>[8x]MGSSHHHHHHSSGRENLYFQGMELLKHLSQRQYIDGEWVESANKNTRDIINPYNQEVIFTVSEGTKEDAERAILAARRAFESGEWSQETAETRGKKVRAIADKIKEHREALARLETLDTGKTLEESYADMDDIHNVFMYFAGLADKDGGEMIDSPIPDTESKIVKEPVGVVTQITPWNYPLLQASWKIAPALATGCSLVMKPSEITPLTTIRVFELMEEVGFPKGTINLILGAGSEVGDVMSGHKEVDLVSFTGGIETGKHIMKNAANNVTNIALELGGKNPNIIFDDADFELAVDQALNGGYFHAGQVCSAGSRILVQNSIKDKFEQALIDRVKKIKLGNGFDADTEMGPVISTEHRNKIESYMDVAKAEGATIAVGGKRPDRDDLKDGLFFEPTVITNCDTSMRIVQEEVFGPVVTVEGFETEQEAIQLANDSIYGLAGAVFSKDIGKAQRVANKLKLGTVWINDFFM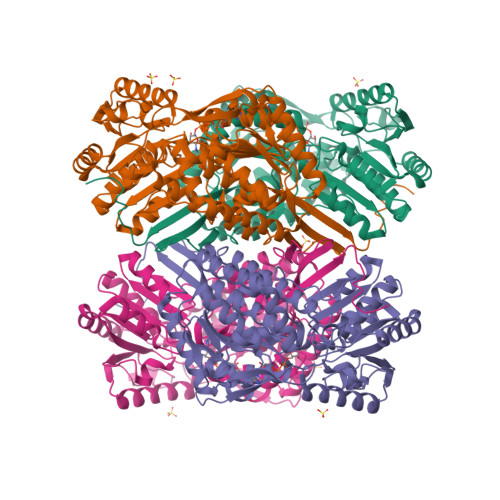YFAQAPWGGYKQSGIGRELGKEGLEEYLVSKHILTNTNPQLVNWFSK> MHHHHHHGGGSENLYFQSPGSAAKGSELSERIESFVE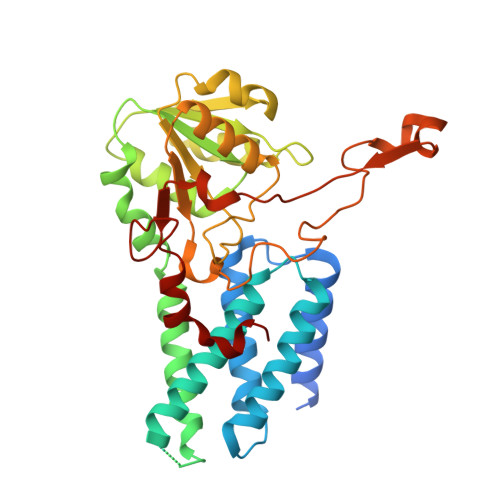TLKRGGGPRSSEEMARETLGLLRQIITDHRWSNAGELMELIRREGRRMTAAQPSETTVGNMVRRVLKIIREEYGRLHGRSDESDQQESLHKLLTSGGLNEDFSFHYAQLQSNIIEAINELLVELEGTMENIAAQALEHIHSNEVIMTIGFSRTVEAFLKEAARKRKFHVIVAECAPFCQGHEMAVNLSKAGIETTVMTDAAIFAVMSRVNKVIIGTKTILANGALRAVTGTHTLALAAKHHSTPLIVCAPMFKLSPQFPNEEDSFHKFVAPEEVLPFTEGDILEKVSVHCPVFDYVPPELITLFISNIGGNAPSYIYRLMSELYHPDDHVL> TQCNVNPVQIPKDWITMHRSCRNSMRQQIQMEVGASLQYLAMGAHFSKDVVNRPGFAQLFFDAASEEREHAMKLIEYLLMRGELTNDVSSLLQVRPPTRSSWKGGV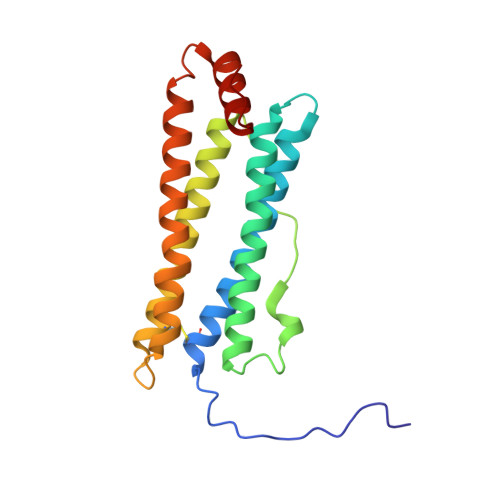EALEHALSMESDVTKSIRNVIKACEDDSEFNDYHLVDYLTGDFLEEQYKGQRDLAGKASTLKKLMDRHEALGEFIFDKKLLGIDV~{tert}-butyl 6-[5-oxidanyl-4-(1,2,3-triazol-1-yl)pyrazol-1-yl]pyridine-3-carboxylate 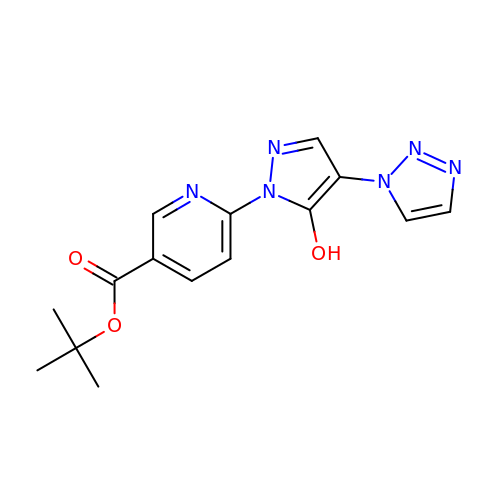| C15 H16 N6 O3 | XGMXSZUIWLEBQB-UHFFFAOYSA-N Toll-like Receptor 3 (TLR3) plays a key role in anti-viral defenses by inducing a potent immune response against double-stranded RNAs (dsRNAs) produced by viral infection. Previous crystallographic studies show that RNA ligand binds to the extracellular domains of TLR3 and induces the formation of a homodimer of TLR326. The charge interaction with the phosphate backbone of the RNA double helix plays the principal role in the interaction. The ligand-binding site involves both the N and C-terminal parts of the TLR3 ectodomain.

Close inspection of the region between the TLR3 dimeric units in the cluster shows that the charge interaction plays a role in the clustering. The closest contact area between the dimeric TLR3 units is composed of the negatively charged N-terminal and the positively charged C-terminal residues of the neighboring ectoTLR3 dimers. To test their role in TLR3 clustering, we made two charge-reversion mutations. The N-terminal mutant, NT-mut had a triple mutation of K117D, K139D and K145D and the C-terminal mutant, CT-mut had a triple mutation of D523K, D524K and E527K of ectoTLR3. For the cryo-EM study, the mutant ectoTLR3 domains were produced and mixed with poly(I:C). The micrographs of the resulting complexes show that the clustering of ectoTLR3 is significantly reduced or entirely blocked by the mutations. The dimeric structure of the mutant ectoTLR3 is still superimposable with that of the wild-type ectoTLR3. Therefore, the effect of the mutation is not due to a conformational change of the TLR3 nor the blocking of TLR3 dimerization. The mutant protein is still able to generate an intracellular signal in response to poly(I:C). This result indicates that the charge interaction between the TLR3 dimers contributes to but is not the predominant factor for clustering under the cellular environment where TLR3s are bound to the membrane.

>ADPKCTVSHEVADCSHLKLTQVPDDLPTNITVLNLTHNQLRRLPAANFTRYSQLTSLDVGFNTISKLEPELCQKLPMLKVLNLQHNELSQLSDDTFAFCTNLTELHLMSNSIQKIDNNPFVDQKNLITLDLSHNGLSSTKLGTQVQLENLQELLLSNNKIQALKSEELDIFANSSLKKLELSSNQIKEFSPGCFHAIGRLFGLFLNNVQLGPSLTEKLCLELANTSIRNLSLSNSQLSTTSNTTFLGLKWTNLTMLDLSYNNLNVVGNDSFAWLPQLEYFFLEYNNIQHLFSHSLHGLFNVRYLNLKRSFTKQSISLASLPKIDDFSFQWLKCLEHLNMEDNDIPGIKSNMFTGLINLKYLSLSNSFTSLRTLTNETFVSLAHSPLHILNLTKNKISKIESDAFSWLGHLEVLDLGLNEIGQELTGQEWRGLENIFEIYLSYNKYLQLTRNSFALVPSLQRLMLRRVALKNVDSSPSPFQPLRNLTILDLSNNNIANINDDMLEGLEKLEILDLQHNNLARLWKHANPGGPIYFLKGLSHLHILNLESNGFDEIPVEVFKDLFELKIIDLGLNNLNTLPASVFNNQVSLKSLNLQKNLITSVEKKVFGPAFRNLTELDMRFNPFDCTCESIAWFVNWINETHTNIPELSSHYLCNTPPHYHGFPVRLFDTSSCKSGRLVPRGSHHHHHH[2x]(2S)-N-[4-[3-cyano-1-[(3,5-dimethyl-1,2-oxazol-4-yl)methyl]indol-5-yl]oxyphenyl]pyrrolidine-2-carboxamide 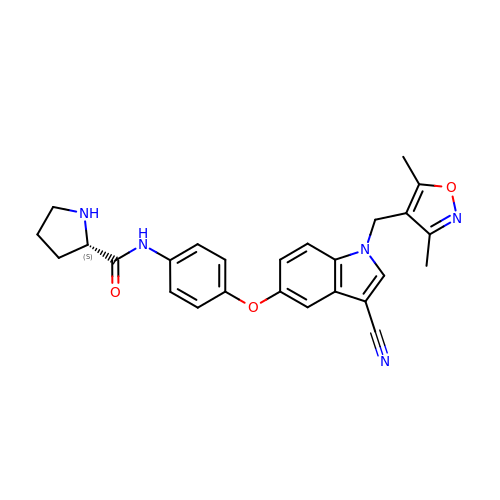| C26 H25 N5 O3 | NDIKFKQBWGMLCA-DEOSSOPVSA-N> MARVQFKQRESTDAIFVHCSATKPSQNVGVREIRQWHKEQGWLDVGYHFIIKRDGTVEAGRDEMAVGSHAKGYNHNSIGVCLVGGIDDKGKFDANFTPAQMQSLRSLLVTLLAKYEGAVLRAHHEVAPKACPSFDLKRWWEKNELVTSDRG;> MNTINIAKNDFSDIELAAIPFNTLADHYGERLAREQLALEHESYEMGEARFRKMFERQLKAGEVADNAAAKPLITTLLPKMIARINDWFEEVKAKRGKRPTAFQFLQEIKPEAVAYITIKTTLACLTSADNTTVQAVASA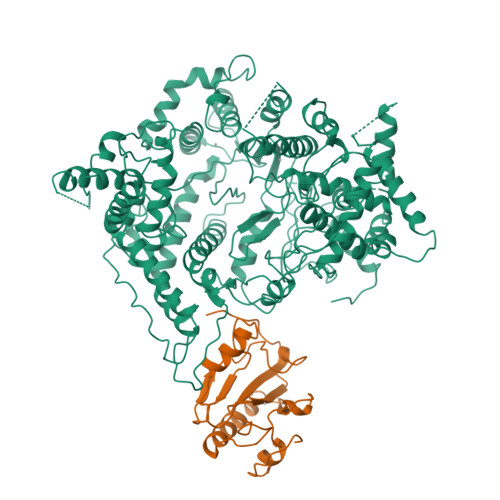IGRAIEDEARFGRIRDLEAKHFKKNVEEQLNKRVGHVYKKAFMQVVEADMLSKGLLGGEAWSSWHKEDSIHVGVRCIEMLIESTGMVSLHRQNAGVVGQDSETIELAPEYAEAIATRAGALAGISPMFQPCVVPPKPWTGITGGGYWANGRRPLALVRTHSKKALMRYEDVYMPEVYKAINIAQNTAWKINKKVLAVANVITKWKHSPVEDIPAIEREELPMKPEDIDMNPEALTAWKRAAAAVYRKDKARKSRRISLEFMLEQANKFANHKAIWFPYNMDWRGRVYAVSMFNPQGNDMTKGLLTLAKGKPIGKEGYYWLKIHGANCAGVDKVPFPERIKFIEENHENIMACAKSPLENTWWAEQDSPFCFLAFCFEYAGVQHHGLSYNCSLPLAFDGSCSGIQHFSAMLRDEVGGRAVNLLPSETVQDIYGIVAKKVNEILQADAINGTDNEVVTVTDENTGEISEKVKLGTKALAGQWLAYGVTRSVTKRSVMTLAYGSKEFGFRQQVLEDTIQPAIDSGKGLMFTQPNQAAGYMAKLIWESVSVTVVAAVEAMNWLKSAAKLLAAEVKDKKTGEILRKRSAVHWVTPDGFPVWQEYKKPIQTRLNLMFLGQFRLQPTINTNKDSEIDAHKQESGIAPNFVHSQDGSHLRKTVVWAHEKYGIESFALIHDSFGTIPADAANLFKAVRETMVDTYESSDVLADFYDQFADQLHESQLDKMPALPAKGNLNLRDILESDFAFA> SRKKIFKPEELRQALMPTLEALYRQDPESLPFRQPVDPQLLGIPDYFDIVKNPMDLSTIKRKLDTGQYQEPWQYVDDVWLMFNNAWLYNRKTSRVYKFCSKLAEVFEQEIDPVMQSLGYCCGRKYEFSPQTLCCYGKQLCTIPRDAAYYSYQNRYHFCEKCFTEIQGENVTLGDDPSQPQTTISKDQFEKKKNDTLDPEPFVD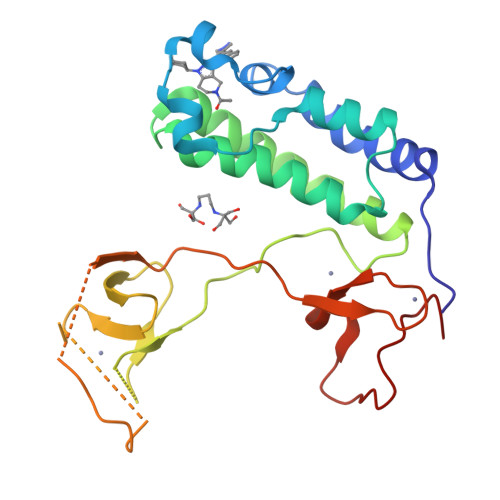CKECGRKMHQICVLHYDIIWPSGFVCDNCL> SNALHLEPLHFLQCHSRNNSPKDLETQLWACAFEPAREEGHSGATSQTVATCGGEAVCVIDCQTGLVLHKYKVPGEEFFSVAWTALTVATQAGHKKRWNMLAAAGLRG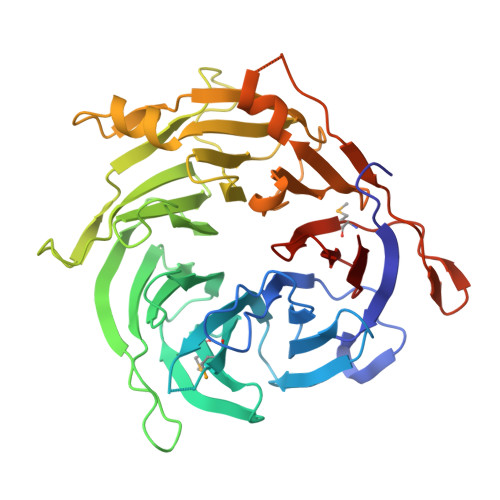MVRLLHVRAGFCCSVIRAHKKAIATLCFSPTHETHLFTASYDKRIILWDIGVPNHDYKFQASQLLTLNCSSVPLRLCPVATCPDSFLLAGCEGGCGCWDVRLDQPQKQRVCEVNFVFSGDSEVSGQRVDGLAFVNEDVVASKGSGQGTIYLWSWSQTWASRGSQSVLPVVILAQLQWSPTSLAYFSLSTCPDKNLVLCGDEEGSVWIYDVEHLLKQPPPLETTLQPPTQILKWPQPVALGQPVTKTMVNTVVANAAFTYLTALTDSNIVSIWRRC> YKDGDQCETSPCQNQGKCKDGLGEYTCTCLEGFEGKNCELFTRKLC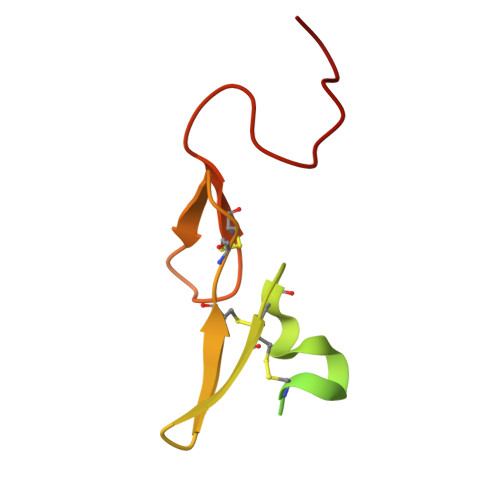SLDNGDCDQFCHEEQNSVVCSCARGYTLADNGKACIPTGPYPCGKQTLER> MGFFDDKQDFLEETFAKYPPEGRRAAIMPLLRRVQQEEGWIRPERIEEIARLVGTTPTEVMGVASFYSYYQFVPTGKYHL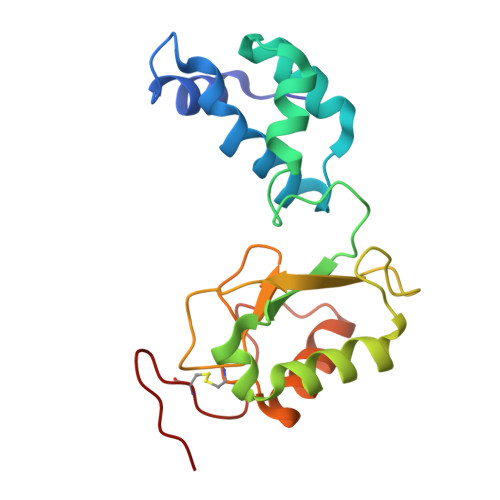QVCATLSCKLAGAEELWDYLTETLGIGPGEVTPDGLFSVQKVECLGSCHTAPVIQVNDEPYVECVTRARLEALLAGLRAGKRLEEIELPGKCGHHVHEVEV>[4x]MHNDKDLSTWQTFRRLWPTIAPFKAGLIVAGIALILNAASDTFMLSLLKPLLDDGFGKTDRSVLLWMPLVVIGLMILRGITSYISSYCISWVSGKVVMTMRRRLFGHMMGMPVAFFDKQSTGTLLSRITYDSEQVASSSSGALITVVREGASIIGLFIMMFYYSWQLSIILVVLAPIVSIAIRVVSKRFRSISKNMQNTMGQVTTSAEQMLKGHKEVLIFGGQEVETKRFDKVSNKMRLQGMKMV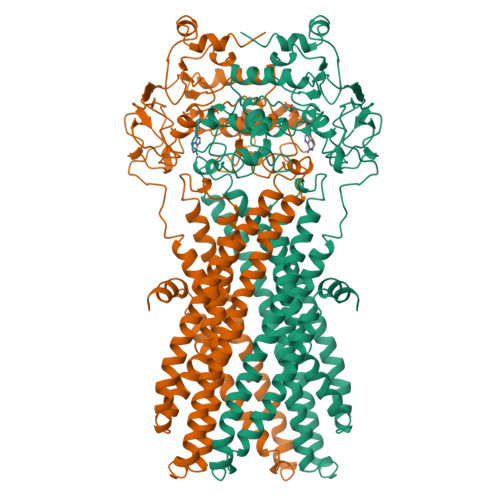SASSISDPIIQLIASLALAFVLYAASFPSVMDSLTAGTITVVFSSMIALMRPLKSLTNVNAQFQRGMAACQTLFAILDSEQEKDEGKRVIDRATGDLEFRNVTFTYPGREVPALRNINLKIPAGKTVALVGRSGSGKSTIASLITRFYDIDEGHILMDGHDLREYTLASLRNQVALVSQNVHLFNDTVANNIAYARTEEYSREQIEEAARMAYAMDFINKMDNGLDTIIGENGVLLSGGQRQRIAIARALLRDSPILILDEATSALDTESERAIQAALDELQKNRTSLVIAHRLSTIEQADEIVVVEDGIIVERGTHSELLAQHGVYAQLHKMQFGQ> MTATVLLEVPFSARGDRIPDAVAELRTREPIRKVRTITGAEAWLVSSYALCTQVLEDRRFSMKETAAAGAPRLNALTVPPEVVNNMGNIADAGLRKAVMKAITPKAPGLEQFLRDTANSLLDNLITEGAPADLRNDFADPLATALHCKVLGIPQEDGPKLFRSLSIAFMSSADPIPAAKINWDRDIEYMAGILENPNITTGLMGELSRLRKDPAYSHVSDELFATIGVTFFGAGVIATGSF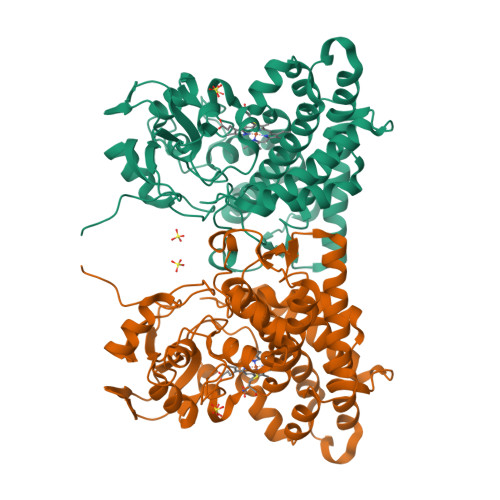LTTALISLIQRPQLRNLLHEKPELIPAGVEELLRINLSFADGLPRLATADIQVGDVLVRKGELVLVLLEGANFDPEHFPNPGSIELDRPNPTSHLAFGRGQHFCPGSALGRRHAQIGIEALLKKMPGVDLAVPIDQLVWRTRFQRRIPERLPVLW>[3x]ADKELKFLVVDDFSTMRRIVRNLLKELGFNNVEEAEDGVDALNKLQAGGFGFIISDWNMPNMDGLELLKTIRADSAMSALPVLMVTA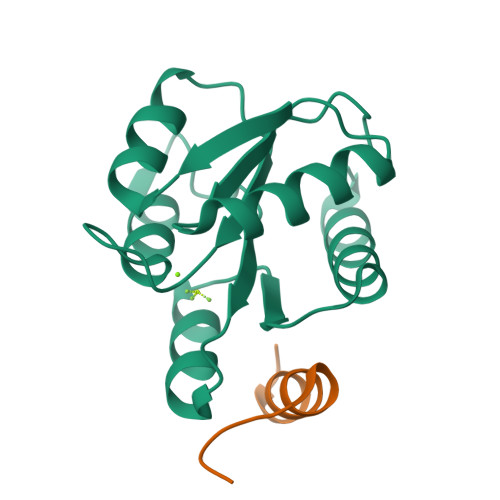EAKKENIIAAAQAGASGYVVKPFTAATLEEKLNKIFEKLGM;>AGVVASQDQVDDLLDSLGF[3x]>SNDIYFNFQRFNETNLILQRDASVSSSGQLRLTNLNGNGEPRVGSLGRAFYSAPIQIWDNTTGTVASFATSFTFNIQVPNNAGPADGLAFALVPVGSQPKDKGGFLGLFDGSNSNFHTVAVEFDTLYNKDWDPTERHIGIDVNSIRSIKTTRWDFVNGENA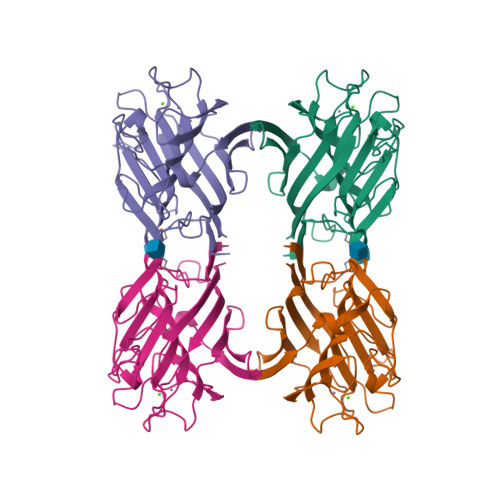EVLITYDSSTNLLVASLVYPSQKTSFIVSDTVDLKSVLPEWVSVGFSATTGINKGNVETNDVLSWSFASKLSDETTSEGLNLANLVLNKIL[4x]> MLRRCCPATLHVAPSTAMVAGVFVNNQKRFLKMAKSAFGFYLARRGQRKFPFLRRPHIKNTHAMNLSAPYFWSFMTAKSQTYFLPEENYITGDWTGKFFVSKLQVYTLQHATSGSTVRVKSFPSVFE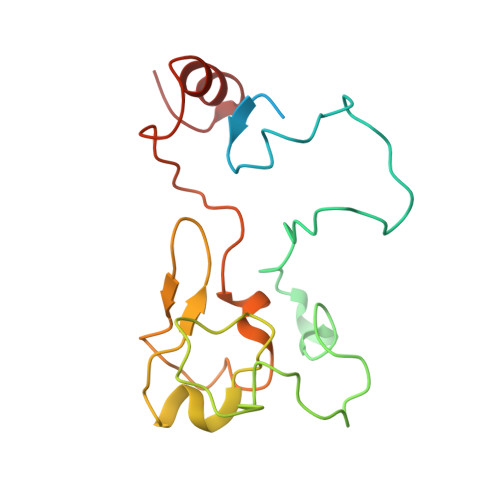LSSPSRWNIGKELNTLTKPRMDLIDEQMLTKKQRLDYVKAGLLPK(2R,3R,4S,5R)-2-(2-azanyl-6-methoxy-purin-9-yl)-5-(hydroxymethyl)oxolane-3,4-diol 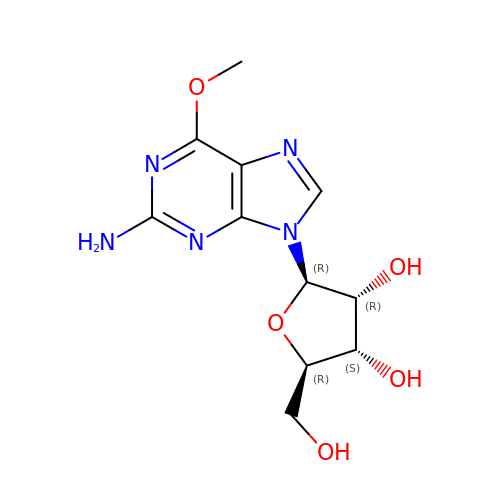| C11 H15 N5 O5 | IXOXBSCIXZEQEQ-KQYNXXCUSA-N>MKELIRKLTEAFGPSGREEEVRSIILEELEGHIDGHRIDGLGNLIVWKGSGEKKVILDAAIDEIGVVVTNVDDKGFLTIEPVGGVSPYMLLGKRIRFENGTIGVVGMEGETTEERQENVRKLSFDKLFIDI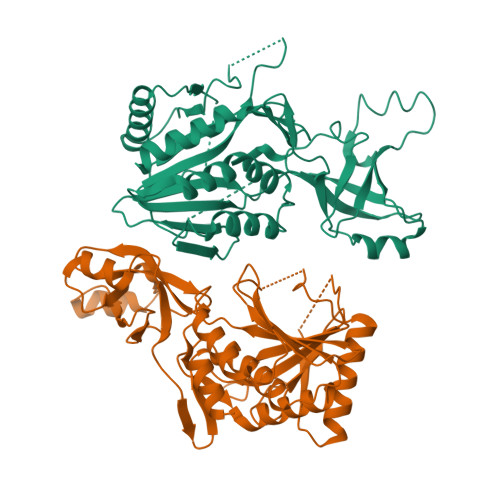GANSREEAQKMCPIGSFGVYDSGFVEVSGKYVSKAMDDRIGCAVIVEVFKRIKPAVTLYGVFSVQEEVGLVGASVAGYGVPADEAIAIDVTDSADTPKAIKRHAMRLSGGPALKVKDRASISSKRILENLIEIAEKFDIKYQMEVLTFGGTNAMGYQRTREGIPSATVSIPTRYVASPSEMIAPDDVEATVDLLIRYLGA[2x]>[2x]QYLLPEAKAQDSDKICVVIDLDETLVHSSFKPVNNADFIIPVEIDGVVHQV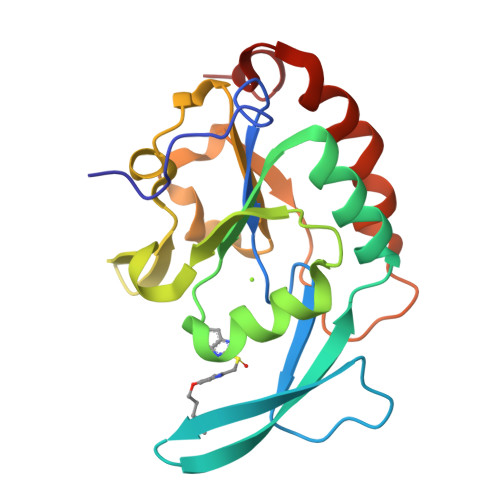YVLKRPHVDEFLQRMGELFECVLFTASLAKYADPVADLLDKWGAFRARLFRESCVFHRGNYVKDLSRLGRDLRRVLILDNSPASYVFHPDNAVPVASWFDNMSDTELHDLLPFFEQLSRVDDVYSVLRQ>MAQFDTEYQRLEASYSDSPPGEEDLLVHVAEGSKSPWHHIENLDLFFSRVYNLHQKNGFTCMLIGEIFELMQFLFVVAFTTFLVSCVDYDILFANKMVNHSLHPTEPVKVTLPDAFLPAQVCSARIQENGSLITILVIAGVFWIHRLIKFIYNICCYWEIHSFYLHALRIPMSALPYCTWQEVQARIVQTQKEHQICIHKRELTELDIYHRILRFQNYMVALVNKSLLPLRFRLPGLGEAVFFTRGLKYNFELILFWGPGSLFLNEWSLKAEYKRGGQRLELAQRLSNRILWIGIANFLLCPLILIWQILYAFFSYAEVLKREPGALGARCWSLYGRCYLRHFNELEHELQSRLNRGYKPASKYMNCFLSPLLTLLAKNGAFFAGSILAVLIALTIYDEDVLAVEHVLTTVTLLGVTVTVCRSFIPDQHMVFCPEQLLRVILAHIHYMPDHWQGNAHRSQT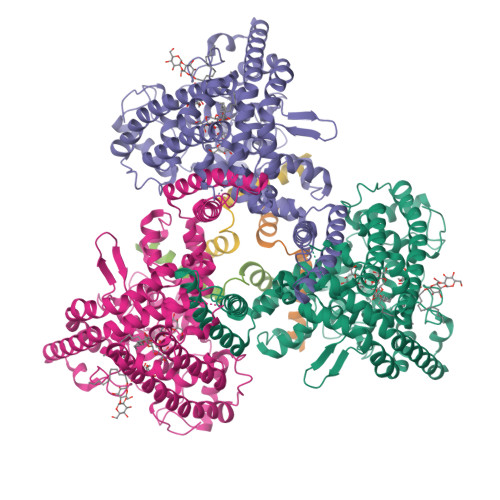RDEFAQLFQYKAVFILEELLSPIVTPLILIFCLRPRALEIIDFFRNFTVEVVGVGDTCSFAQMDVRQHGHPQWLSAGQTEASVYQQAEDGKTELSLMHFAITNPGWQPPRESTAFLGFLKEQVQRDGAAASLAQGGLLPENALFTSIQSLQSESEPLSLIANVVAGSSCRGPPLPRDLQGSRHRAEVASALRSFSPLQPGQAPTGRAHSTMTGSGVDARTASSGSSVXXXXXXXXXXXXXXXXXXXXXXXXXXXXXXXXXXXX[6x]N-(1-{[(3-tert-butylbenzoyl)amino]methyl}cyclohexyl)-2,1-benzoxazole-4-carboxamide 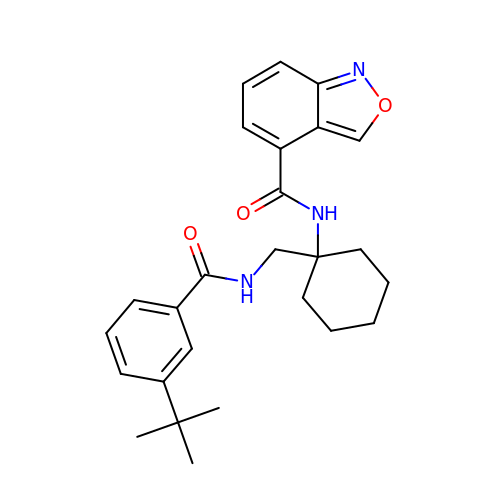| C26 H31 N3 O3 | HBQXFVMSOMIMBK-UHFFFAOYSA-N>[2x]MTMDE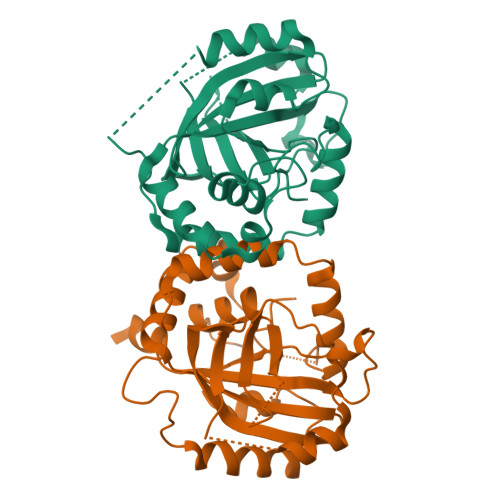QQSQAVAPVYVGGFLARYDQSPDEAELLLPRDVVEHWLHAQGQGQPSLSVALPLNINHDDTAVVGHVAAMQSVRDGLFCLGCVTSPRFLEIVRRASEKSELVSRGPVSPLQPDKVVEFLSGSYAGLSLASRRCDDVEQATSLSGSETTPFKAVALCSVGRRRGTLAVYGRDPEWVTQRFPDLTAADRDGLRAQWQRCGSTAVDASGDPFRSDSYGLLGNSVDALYIRERLPKLRYDKQLVGVTERESYVKA>MSNEAHTLVTPEGNVIDIQGASQENGANAIIYPRHGGENQLFFIDKQIGWIISVFSRKALTVKENMHDIVQSDYCSLSRQQ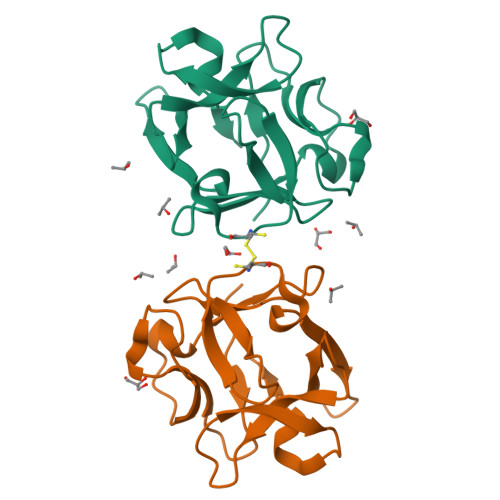WIFEDNPDGTTIIRCYENPELVLSVTGNIDKVCLSPFTREAHQLWRIE[3x]>[6x]MFYINSKYKIDLDKIMTKMKNKSVINIDDVDDEE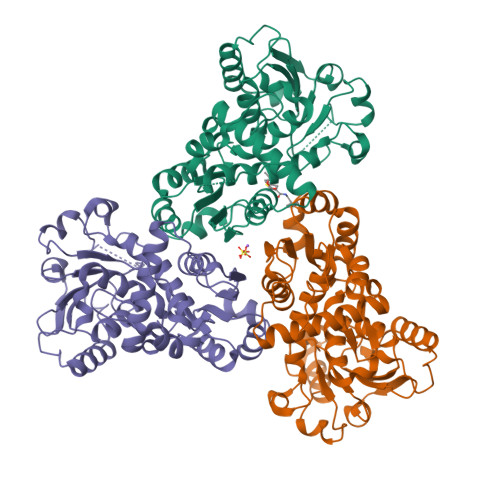LLAILYTSKQFEKILKNNEDSKYLENKVFCSVFLEPSTRTRCSFDAAILKLGSKVLNITDMNSTSFYKGETVEDAFKILSTYVDGIIYRDPSKKNVDIAVSSSSKPIINAGNGTGEHPTQSLLDFYTIHNYFPFILDRNINKKLNIAFVGDLKNGRTVHSLSKLLSRYNVSFNFVSCKSLNIPKDIVNTITYNLKKNNFYSDDSIKYFDNLEEGLEDVHIIYMTRIQKERFTDVDEYNQYKNAFILSNKTLENTRDDTKILHPLPRVNEIKVEVDSNPKSVYFTQAENGLYVRMALLYLIFSSTSSAWSHPQFEK>[3x]AQVINTF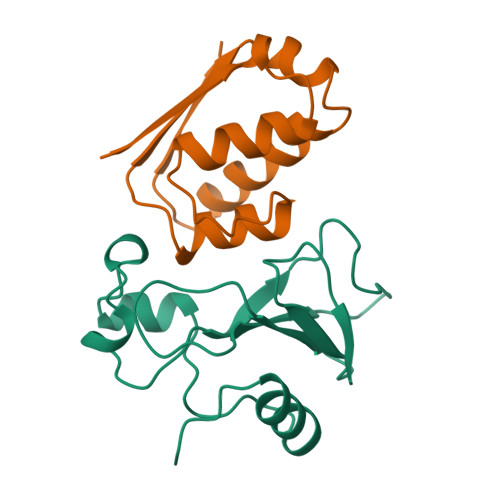DGVADYLQTYHKLPDNYITASEAQALGWVASKGNLADVAPGKSIGGDIFSNREGKLPGKSGRTWREADINYTSGFRNSDRILYSSDWLIYKTTDHYQTFTKIR;>[3x]MKKAVINGEQIRSISDLHQTLKKELALPEYYGENLAALWDCLTGWVEYPLVLEWRQFEQSKQLTENGAESVLQVFREAKAEGCDITIILS> SYTRSEEIESLEQFHMATASSLIHKQMCSIVYTGPLKVQQMKNFIDSLVASLSAAVSNLVKILKDTAAIDLETRQKFGVLDVASKRWLVKPSAKNHAWGVVETHARKYHVALLEHDEFGIITCDNWRRVAVSSESVVYSDMAKLRTLRRLLKDGEPHVSSAKVVLVDGVPGCGKTKEILSRVNFEEDLILVPGRQAAEMIRRRANASGIIVATKDNVRTVDSFLMNYGKGARCQFKRLFIDEGLMLH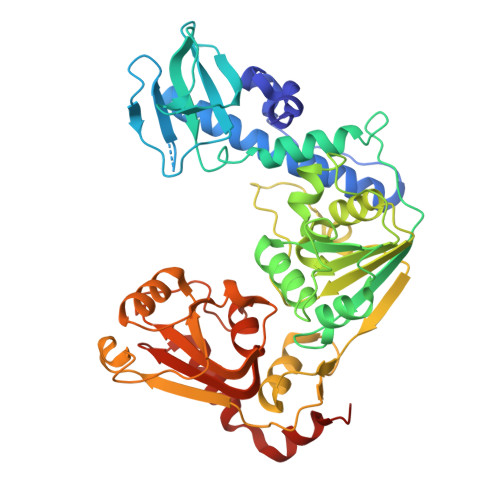TGCVNFLVEMSLCDIAYVYGDTQQIPYINRVTGFPYPAHFAKLEVDEVETRRTTLRCPADVTHFLNQRYEGHVMCTSSEKKSVSQEMVSGAASINPVSKPLKGKILTFTQSDKEALLSRGYADVHTVHEVQGETYADVSLVRLTPTPVSIIARDSPHVLVSLSRHTKSLKYYTVVMDPLVSIIRDLERVSSYLLDMYKVDAGTQ> AMRTIYVIGIGTGSPEFLTLQAISGLRHAQAIVALDKGEQKSDLLALRQKIVDTHAPGTPIYAVTDPERDRNPDNYEEEVRRWHAERAHLLASTIRERTPDDGAVAFLVWGDPSLYDSTLRIIEHMRNLEDLHADVKVIPGITAVQVLTAEHGILINRIGEAI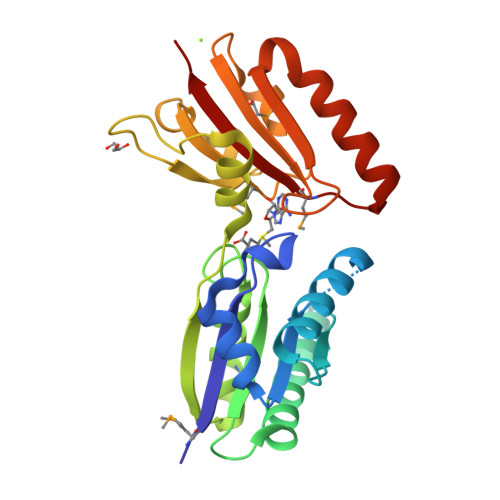HITTGRNLPETSAKDRRNCVVMLDGKTAWQDVATEHTYMWWGAFLGTEQQVLRKGYVHEIGAQVAELKQQLRTEHGWIMDTYLLRELD Deacylation of Cer to sphingosine and subsequent phosphorylation by sphingosine kinase lead to the formation of sphingosine-1-phosphate (S1P), whose irreversible degradation by S1P lyase (SPL) terminates sphingolipid metabolism. SPL (EC 4.1.2.27) is a pyridoxal 5′-phosphate (PLP)-dependent enzyme bound to the endoplasmic reticulum membrane through an N-terminal sequence, with the catalytic domain facing the cytosol. The protein is a tight dimer and belongs to the Fold Type I family. The active site is formed by residues from both subunits and comprises an Y-shaped channel whose distal part is largely hydrophobic.

To confirm the soundness of our virtual screening campaign, we solved the crystal structures of unbound hSPL and AfuSPL at 1.8 Å and 3.5 Å resolution, respectively. The structure of AfuSPL was solved at low resolution. Structural superposition with the human protein results in a RMSD of 0.82 Å (between 412 Cα pairs). Notably, the AfuSPL structure displays a structured N-terminal region, consisting of a long helix that is not observed in hSPL, although its presence in hSPL is predicted by AlfaFold50. This helix is positioned near the active site access cleft and, at least in the soluble construct, is much more flexible for the human protein compared to the fungal enzyme. Moreover, AfuSPL has an insertion of six residues in the C-terminal region that may also alter the dynamics of the substrate binding cleft. On the other hand, no significant differences are observed at the active site level, where all the residues likely involved in substrate binding are conserved. Finally, it must be noted that the position of the additional N-terminal helix that is observed in the AfuSPL structure suggests that the protein binds to the membrane with an orientation that places the active site entrance on the opposite side with respect to the membrane surface. In particular, the N-terminus helix, that is structured in AfuSPL and disordered in hSPL, partially covers the access to the binding poket and provides additional hydrophobic residues to stabilise the binding of lipophilic compounds, and this may account for the higher interaction of AfuSPL with ANS. A clear explanation to these data is not currently available, but we could speculate that this is due to either the structured N-terminal helix in AfuSPL, which could increase binding affinity by partly closing the cleft and preventing ligand dissociation, or to the increased flexibility of the regions allowing the access to the active site in AfuSPL, which could favour the adaptation of the ligands to the active site cleft.

>MPGVRGQVDKQVSTAIENIENKLVASGPGVTRYLTLPQTGWTPEQIRTELDKLANMEHTRWEDGRVSGAVYHGGQDLLKLQTEAFGQFGVANPIHPDVFPGVRKMEAEVVAMVLALFNAPSDGAGVTTSGGTESILMACLAARQKAFTERGVKEPEIIIPDTAHAAFYKACNYFGMKLHRVPCPAPEYKVDIAAVRRLINPNTVLLVGSAPNFPHGIVDDIPALSRLATKYKIPLHVDCCLGSFVIAFLKKAGFPSPYEEEGGFDFRLPGVTSISVDTHKYGFAPKGNSVLLYRNKTYRSYQYFIYPDWSGGVYASPSVAGSRPGALIAGCWASLMSVGETGYINSCLEIIGAAKKFEASIKEHPVLSKNLGIVGKPMVSVVAFQSQNGAVDIYDVADGLSAKGWHLNALQSPPAIHVAFTIPTAAAVEKLTTDLVETVEKELEKAEERKRQGKSYVLKRGDTSALYGVAGSLPDKSIVSRLAEGFLDTLYKAGGGSHHHHHH[2x]3-IODO-TYROSINE | C9 H10 I N O3 | 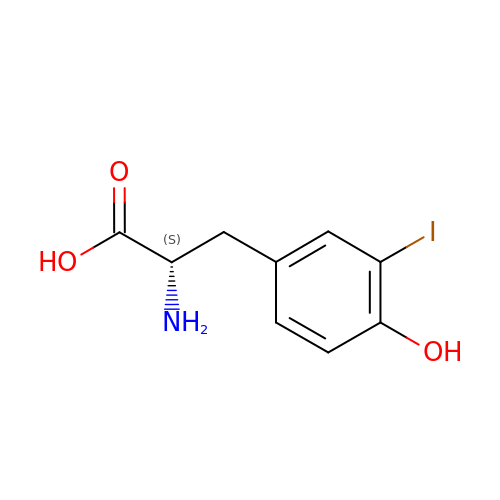UQTZMGFTRHFAAM-ZETCQYMHSA-N> GAMAVTVPVDVVMVIDQSSSMGGQNIARLKSAIASGQRFVKKMLPKGMATEGVRIALVSYDHEPHRLSDFTKDTAFLCQKIRALTPIWGTHTQGGLKMARNIMATSTAVDKHIILMSDGLATEQYPVKNVTTADFIGETGNANDPIDLVIQGAINFPTNYVSNNPSTPLTPNYPTHSSKVGRRNLPESKFDYSNLSARITFDGVAGALVYEPRFPHPY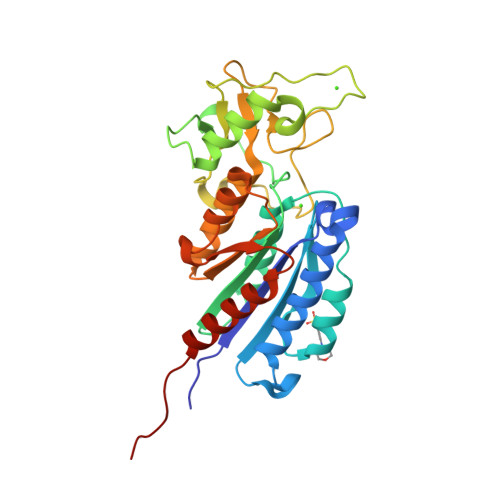YYYFPCNAAINEAQFAKNSGYTIHTIGYDLGDFALANNSLKLTATDENHFFTATPANLAAAFDNIAQTINIGIQRGEVTDFVA> PSKTSNTIRVFLPNKQRTVVRVRNGMSLHDCLMKK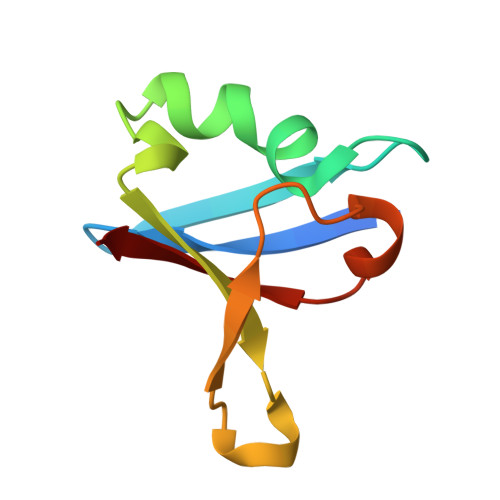LKVRGLQPECCAVFRLLHEHKGKKARLDWNTDAASLIGEELQVDFL> C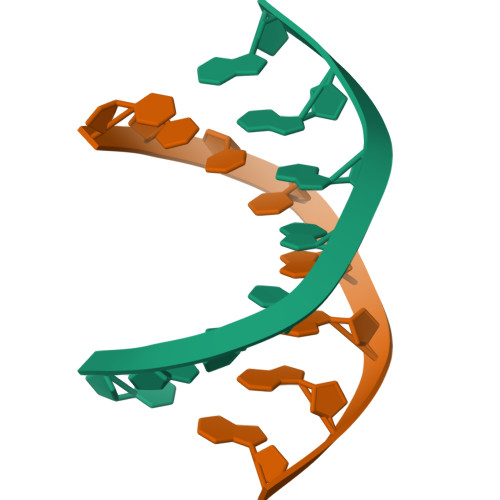CCTAGGG>[2x]MSLDIQSLDIQCEELSDARWAELLPLLQQCQVVRLDDCGLTEARCKDISSALRVNPALAELNLRSNELGDVGVHCVLQGLQTPSCKIQKLSLQNCCLTGAGCGVLSSTLRTLPTLQELHLSDNLLGDAGLQL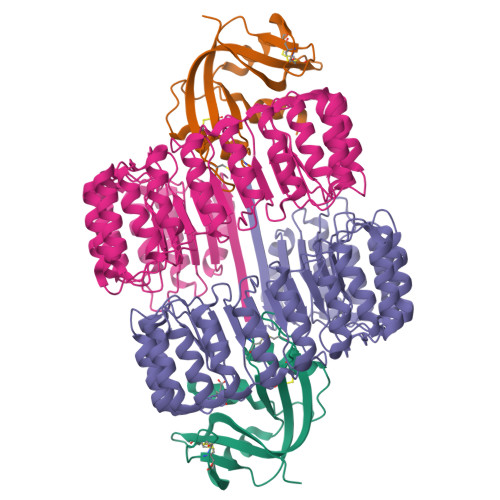LCEGLLDPQCRLEKLQLEYCSLSAASCEPLASVLRAKPDFKELTVSNNDINEAGVRVLCQGLKDSPCQLEALKLESCGVTSDNCRDLCGIVASKASLRELALGSNKLGDVGMAELCPGLLHPSSRLRTLWIWECGITAKGCGDLCRVLRAKESLKELSLAGNELGDEGARLLCETLLEPGCQLESLWVKSCSFTAACCSHFSSVLAQNRFLLELQISNNRLEDAGVRELCQGLGQPGSVLRVLWLADCDVSDSSCSSLAATLLANHSLRELDLSNNCLGDAGILQLVESVRQPGCLLEQLVLYDIYWSEEMEDRLQALEKDKPSLRVIS;>MKESRAKKFQRQHMDSDSSPSSSSTYCNQMMRRRNMTQGRCKPVNTFVHEPLVDVQNVCFQEKVTCKNGQGNCYKSNSSMHITDCRLTNGSRYPNCAYRTSPKERHIIVACEGSPYVPVHFDASVEDST[2x]> 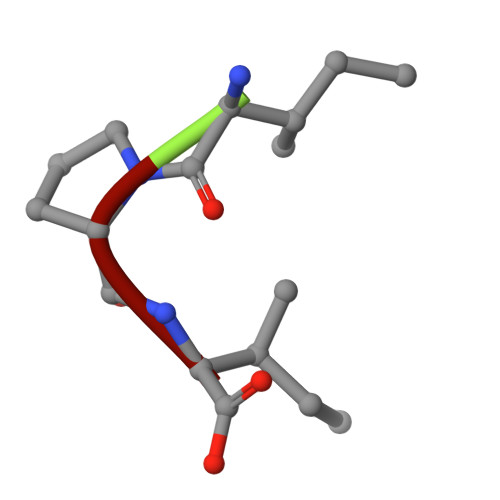IPI FtsEX comprises a cell division-regulating integral membrane protein (FtsX) and a cytoplasmic ATPase (FtsE) that resembles an ATP-binding cassette (ABC) transporter. Hydrolysis causes a conformational change that is transmitted through the membrane via FtsX, an integral membrane protein with two extracellular loops (ECLs), denoted the large (ECL1) and small (ECL2) loops. The folded structure (residues 57 to 166) reveals a central core composed of a four-stranded antiparallel β-sheet (β1, β6, β4, and β5) and two helices (α1 and α3), an α-helical lobe (residues 107 to 135) harboring the α2 helix, and an extended β-hairpin (β2 and β3). The helical lobe mediates a physical interaction with the peptidoglycan hydrolase PcsB via the coiled-coil domain of PcsB (PscBCC).

Three different structures, with resolutions ranging from 2.0 to 2.3 Å, were solved by X-ray crystallography, each in the presence of a different detergent. The detergents used were dodecyltrimethylammonium chloride (detergent 1 [D1]), n-undecyl-β-d-maltoside (detergent 2 [D2]), and n-decyl-β-d-maltoside (detergent 3 [D3]). In all cases, two independent protein molecules are present in the asymmetric unit, arranged in such a way as to keep hydrophobic residues from their α-helical lobes buried. Different conformations were observed for the β-hairpin and the helical lobe among the six structures, depending on the presence and identity of the detergent molecule bound to FtsXECL1. In any case, the crystal structures suggest that changes in the protein backbone and side chains of the helical lobe occur when a detergent ligand is bound. These changes create a cavity in which the detergent molecules insert, with a large part of the helical lobe (from Q111 to E127) affected by the interaction with detergent. Residues Y112, W123, E127, and F126 are strongly perturbed upon detergent ligand binding, with the hydroxyl moiety of Y112 interacting with carboxylate of E127. Changes in W123 and F126 stabilize the hydrophobic region of detergent 1. Full stabilization of the hydrophobic tail of the detergents is completed by the same hydrophobic residues (W123 and F126) but from a symmetry-related molecule. Although a physiological role for detergent binding to the helical lobe is unknown, many of these same residues are important for the interaction with PcsB (see below).

>KLATDIENNVRVVVYIRKDVEDNSQTIEKEGQTVTNNDYHKVYDSLKNMSTVKSVTFSSKEEQYEKLTEIMGDNWKIFEGDANPLYDAYIVEANAPNDVKTIAEDAKKIEGVSEVQD[2x]> MGILQANRVLLSRLLPGVEPEGLTVRHGQFHQVVIASDRVVCLPRTAAAAARLPRRAAVMRVLAGL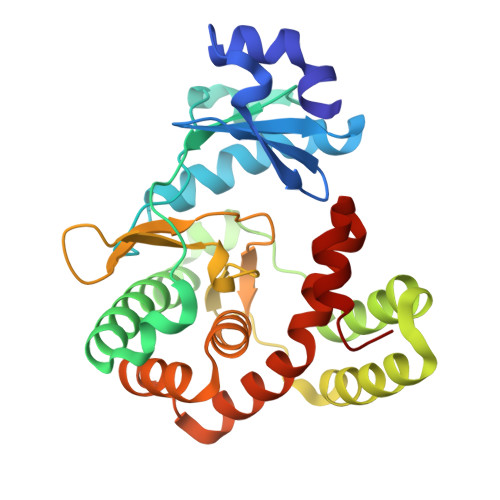DLGCRTPRPLCEGSAEGAVELPFLVLSRVPGAPLEADALEDSKVAEVVAAQYVTLLSGLASAGADEKVRAALPAPQGRWRQFAADVRAELFPLMSDGGCRQAERELAALDSLPDITEAVVHGNLGAENVLWVRDDGLPRLSGVIDWDEVSIGDPAEDLAAIGAGYGKDFLDQVLTLGGWSDRRMATRIATIRATFALQQALSACRDGDEEELADGLTGYR>[10x]MSRTTPYRLDDQIGFILRQANQRYAALFANGIGNGLT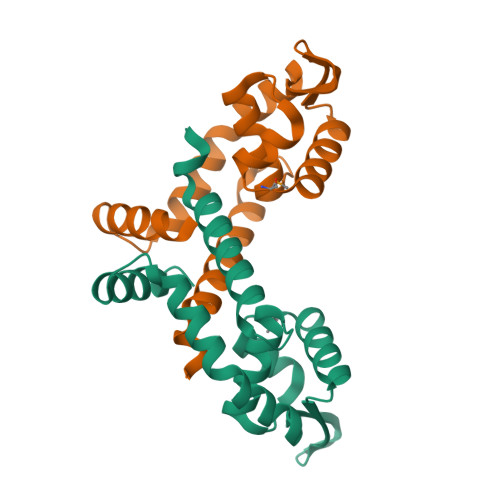PTQWAALVRLGETGPCPQNQLGRLTAMDAATIKGVVERLDKRGLIQRSADPDDGRRLLVSLSPAGRAELEAGLAAAREINRQALAPLSLQEQETLRGLLARLI>[4x]MSKLSVFFIFLFCSIATAAESLPDLKIEKLDEGVYVHTSFEEVNGWGVVPKHGLVVLVNAEAYLIDTPFTAKDTEKLVTWFVERGY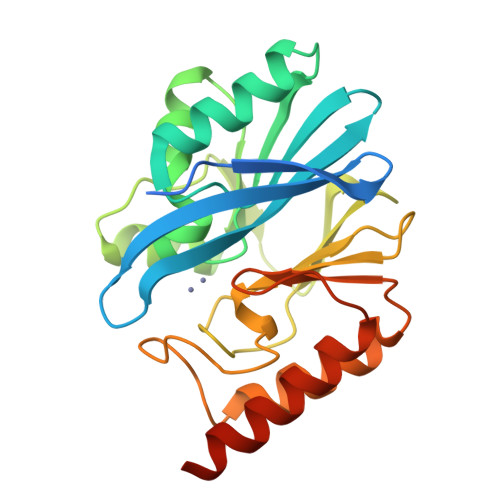KIKGSISSHFHSDSTGGIEWLNSRSIPTYASELTNELLKKDGKVQATNSFSGVNYWLVKNKIEVFYPGPGHTPDNVVVWLPERKILFGGCFIKPYGLGNLGDANIEAWPKSAKLLKSKYGKAKLVVPSHSEVGDASLLKLTLEQAVKGLNESKKPSKPSN> AFSRPGLPVEYLQVPSASMGRDIKVQFQGGGPHAVYLLDGLRAQDDYNGWDINTPAFEEYYQSGLSVIMPVGGQSSFYTDWYQPSQSNGQNYTYKWETFLTREMPAWLQANKGVSPTGNAAVGLAMSGGSALILAAYYPQQFPYAASLSGFLNPSEGWWPTLIGLAMNDSGGYNANSMWGPSSDPAWKRNDPMVQIPRLVANNTRIWVYCGNGTPSDLGGDNIPAKFLEGLTLRTNQTFRDTYAADGGRNGVFNFPPNGTHSWPYWNE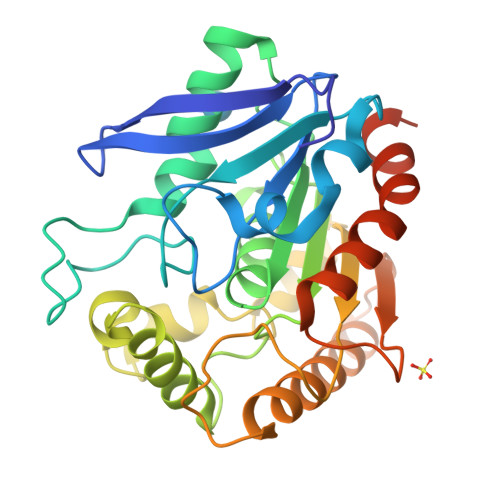QLVAMKADIQHVLNGATPPAAPAAPAAHHHHHH> QRCRHQFQTQQRLRACQRVIQR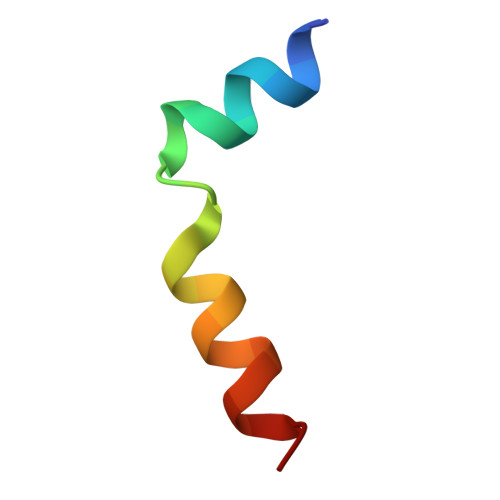WSQ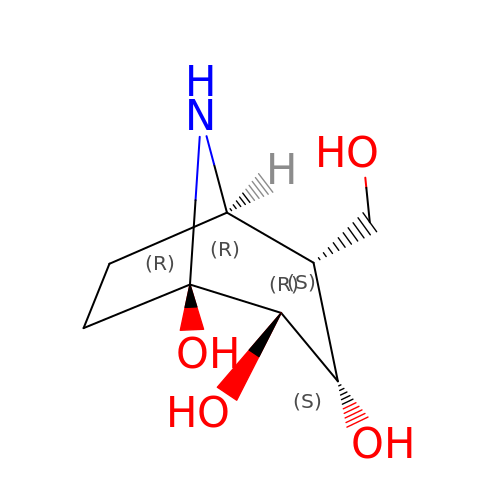(1~{R},2~{S},3~{S},4~{R},5~{R})-4-(hydroxymethyl)-8-azabicyclo[3.2.1]octane-1,2,3-triol | C8 H15 N O4 | NLSPHUUFXPUPJJ-GWVFRZDISA-N> ETVPVKLKPGMDGPKVKQWPLTEEKIKALVEICTEMEKEGKISKIGPENPYNTPVFAIKKKDSTKWRKLVDFRELNKRTQDFWEVQLGIPHPAGLEKKKSVTVLDVGDAYFSVPLDEDFRKYTAFTIPSINNETPGIRYQYNVLPQGWKGSPAIFQSSMTKILEPFRKQNPDIVIYQYMDDLYVGSDLEIGQHRTKIEELRQHLLRWGLTTPDKKHQKEPPFLWMGYELHPDKWTVQPIVLPEKDSWTVNDIQKLVGKLNWASQIYPGIKVRQLCKLLRGTKALTEVIPLTEEAELELAENREILKEPVHGVYYDPSKDLIAEIQKQGQGQWTYQIYQEPFKNLKTGKYARMRGAHTNDVKQLTEAVQKITTESIVIWGKTPKFKLPIQKETWET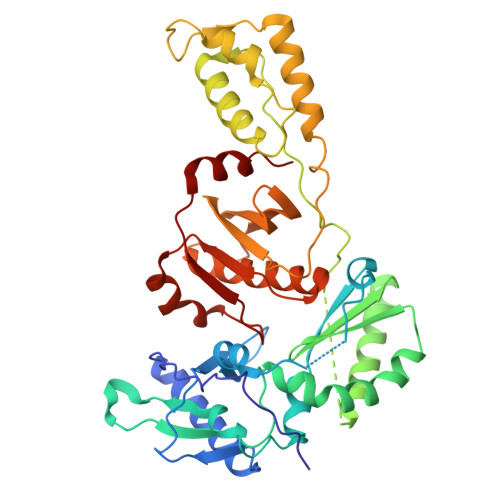WWTEYWQATWIPEWEFVNTPPLVKLWYQLEK~{N}-[3-fluoranyl-4-(4-methylpiperazin-1-yl)phenyl]-4-pyrazolo[1,5-b]pyridazin-3-yl-pyrimidin-2-amine 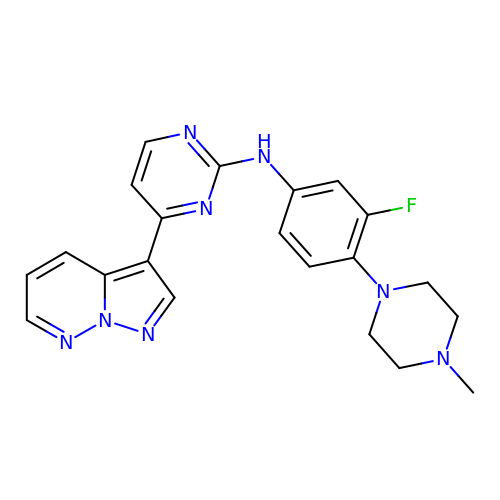| C21 H21 F N8 | YKOSORGDWOWAJE-UHFFFAOYSA-N>[2x]SAAIGLFYGTQTGKTESVAEIIRDEFGNDVVTLHDVSQAEVT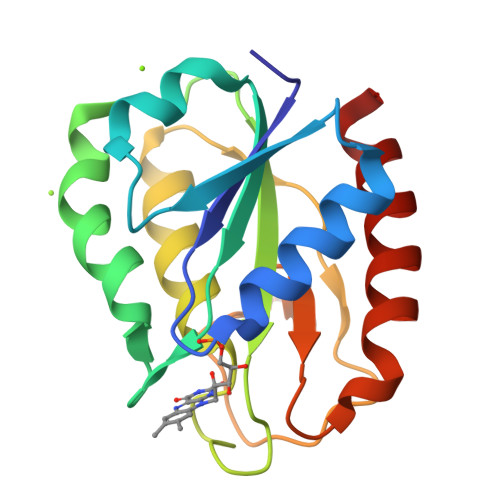DLNDYQYLIIGCPTWNIGELQSDWEGLYSELDDVDFNGKLVAYFGTGDQIGYADNFQDAIGILEEKISQRGGKTVGYWSTDGYDFNDSKALRNGKFVGLALDEDNQSDLTDDRIKSWVAQLKSEFGL>[2x]SSSFDKGKYKKGDDASYFEPTGPYLMVNVTGVDGKGNELLSPHYVEFPIKPGTTLTKEKIEYYVEWALDAT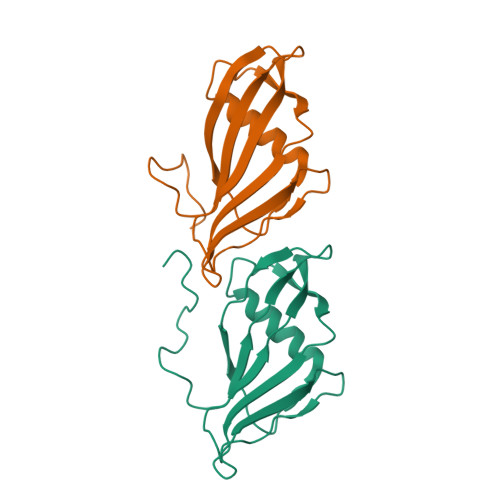AYKEFRVVELDPSAKIEVTYYDKNKKKEETKSFPITEKGFVVPDLSEHIKNPGFNLITKVVIEKK>TRDQNGTWEMESNENFEGYMKALDIDFCTRKIAVRCTQTKVIDQDGDNFKDKTTSTFRNYDVDFTVGVEFDEYTKSLDNRHVKALVTWE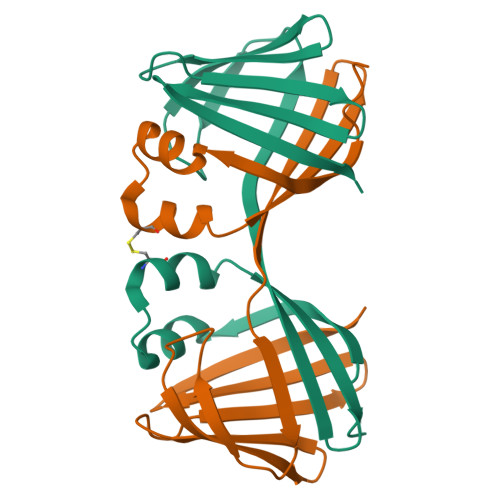GDVLVCVQKGEKENRGWKKWIEGDKLYLELTCGDQVCRQVFKKK[2x]> APVRSLNCT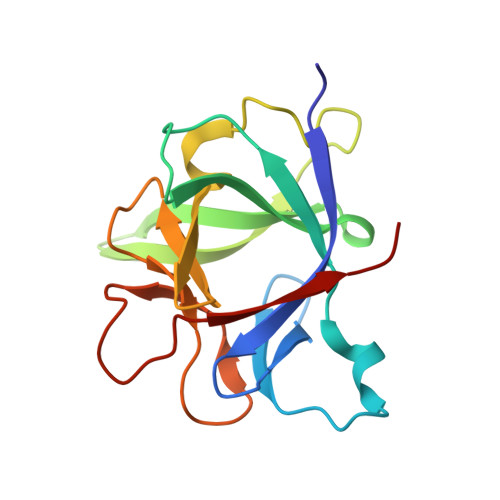LRDSQQKSLVMSGPYELKALHLQGQDMEQQVVFSMSFVQGEESNDKIPVALGLKEKNLYLSCVLKDDKPTLQLESVDPKNYPKKKMEKRFVFNKIEINNKLEFESAQFPNWYISTSQAENMPVFLGGTKGGQDITDFTMQFVSS>[6x]MGKACLQNGTRLLRADGSEVLVEDVQEGDQLLGPDGTSRTASKIVRGEERLYRIKTHEGLEDLVCTHNHILSMYK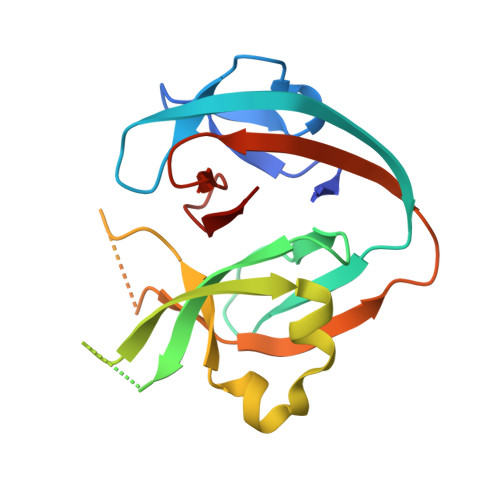ERFGREGAHSPSAGTSLTESHERVDVTVDDFVRLPQQEQQKYKLFRSTDFVRREQPSASKLATLLHINSIELEEEPTKWSGFVVDKDSLYLRYDYLVLHNS> MGEPQQVSALPPPPMQYIKEYTDENIQEGLAPKPPPPIKDSYMMFGNQFQCDDLIIRPLESQGIERLHPMQFDHKKELRKLNMSILINFLDLLDILIRSPGSIKREEKLEDLKLLFVHVHHLINEYRPHQARETLRVM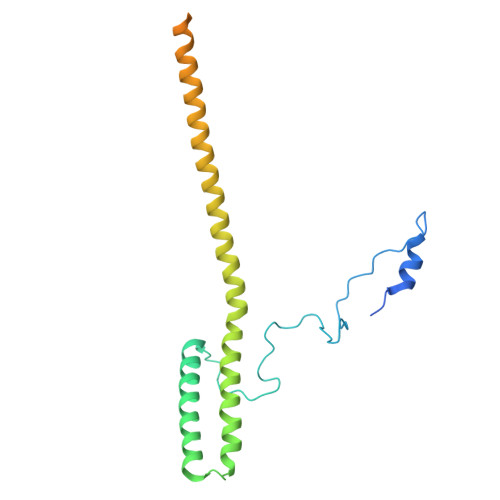MEVQKRQRLETAERFQKHLERVIEMIQNCLASLPDDLPHSEAGMRVKTEPMDADDSNNCTGQNEHQRENSGHRRDQIIEKDAALCVLIDEMNERP> MGSSHHHHHHSSGPQQGLRYEAETATLKGKFRKKEHRKQTGVFFDKGKGNSIEWNISTGLAQVYALRFKYMNTTGKPMPVLMKFIDSKGVVLKEDILTFPETPDKWKMMSTTTGTFINAGHYKVLLSAENMDGLAFDALDI

BT0996 protein acts in the initial stages of the RG-II depolymerisation, where its two catalytic modules remove the terminal monosaccharides from RG-II side chains A and B. BT0996 is modular and has three putative carbohydrate-binding modules (CBMs) for which the roles in the RG-II degradation are unknown. Here, we present the characterisation of the module at the C-terminal domain, which we designated BT0996-C. The high-resolution structure obtained by X-ray crystallography reveals that the protein displays a typical β-sandwich fold with structural similarity to CBMs assigned to families 6 and 35. In line with this, carbohydrate microarrays and microscale thermophoresis show the ability of BT0996-C to bind α1-4-linked polygalacturonic acid, and that electrostatic interactions are essential for the recognition of the anionic polysaccharide. The results support the hypothesis that BT0996-C may have evolved to potentiate the action of BT0996 catalytic modules on the complex structure of RG-II by binding to the polygalacturonic acid backbone sequence.

The crystal structure of BT0996-C with the N-terminal His-tag was determined at 1.65 Å resolution by molecular replacement using, as phasing model, the preliminary 2.3 Å resolution structure of the C-terminal His-tag construct, solved by Se-SAD. The final refined high-resolution structure contained one molecule of BT0996-C in the asymmetric unit, consisting of 122 amino acid residues of the wild-type protein and an additional nine residues of the N-terminal tag. BT0996-C displays a distorted β-sandwich, composed of two β-sheets connected by loops. β-Sheet A includes β-strands 1, 3, 4, 11, 6 and 9, whereas β-sheet B comprises β-strands 2, 5, 10, 7 and 8. The structural calcium ion, highly conserved in many lectins and CBM families (Correia et al., 2010, Sainz-Polo et al., 2014), is positioned near β-1, β-11 strands and H1 helix. This metal ion is coordinated by Glu21 Oε1, Glu23 Oε1 and Oε2, Asp137 Oδ1, the backbone carbonyls of Asp137, Thr40, and one water molecule, in an octahedral geometry confirmed by the Check My Metal server (Zheng et al., 2014). A striking feature of BT0996-C is its high content in positively charged residues (15 Lys, 2 His and 4 Arg), representing almost 20 % of the protein composition, resulting in a theoretical isoelectric point (pI) of 9.43. This feature confers a prominent broad positive patch to the electrostatic surface of the BT0996-C protein, which includes both β-sheets and the loops that connect them. Instead, in the 3D structure here reported, a 2-methyl-2,4-pentanediol (MPD) molecule present in the crystallisation solution could be modelled, establishing CH–π interactions to His36 and water-mediated hydrogen bonds to Gly133 O and Thr73 Oγ1 from β-sheets 3 and 4, near the loop region.>MAHHHHHHMRITVDRSQFFKSLGRVHRVVERRNTVPILSNVLIDAENGSVQLKATDLDLEVTESFTVNIEKAGAITVPAYLLYDIVRKLPDGSEIVLSVDENQASAMSIVSGCTHFQLQCLPKIDFPESLPGQFGCRFFLSASKLKHLLDCTQFAISTEETRYYLNGIYFHIVHDDVLKLRLVATDGHRLAQVDMEAPSGVDGMPGVIIPRKAVGELQKLLSEEIDGDVCIELSETKIRFSLGSVVFTSKLVDGTFPDYQRV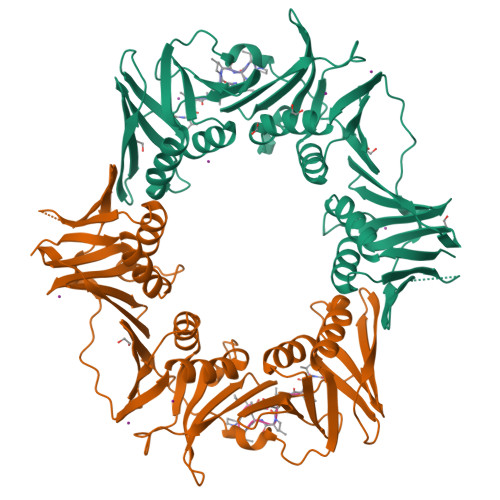IPLGNDRKLIVNRQDFSSAVDRVSTISNDRGRAVKLTIEHGQLKLVVNNPDSGSAEDQLAATYTSEPLEIGFNSRYLLDIAGQLSSDEMVFMLSDAVAPALIRDNNNAEVLYVLMPVRV[2x];>XVPTLPLVPXG[2x]Riboswitches are gene regulatory elements that are frequently found in the 5′-untranslated regions of bacterial mRNAs (1–6). Only very recently, the nadA RNA motif has been assigned to function as a riboswitch which regulates the expression of genes involved in biosynthesis of the enzyme cofactor nicotinamide adenine dinucleotide (NAD+). Although the cofactor is ubiquitous, this riboswitch appears to be rather rare and has the special feature of a tandem aptamer architecture. Here, we report crystal structures of the first, as well as the second domain of the NAD+ riboswitch, both individually bound to NAD+.

For the structural studies on domain 2 of the NAD+ riboswitch, we used the sequence information from Acidobateriaceae bacterium KBS83. Though attempts to crystallize the full-length NAD+ riboswitch in the presence of NAD+ were unsuccessful, we did succeed in generating crystals of domain 2 alone in complex with NAD+ (832GAAA-D2/NAD+), diffracting at a resolution of 2.1 Å. The structure was named as 832GAAA-D2/NAD+, the space group of 832GAAA-D2/NAD+ was P3221, in which each asymmetric unit contain one molecule. Also, the ligand NAD+ is bound similarly to domain 1, positioned at the intersection of the north terminus of stem P1 and the junction J1. All stacking and hydrogen bonding interactions are retained and the three octahedrally coordinated Mg2+ ions are also present with a similar coordination pattern to NAD+ and the nucleotides in the binding pocket of 832GAAA-D2. The long double helical arrangement of stem P1a and P1b, however, shows clear distinctions originating from the altered nucleoside composition of J2 in 832GAAA-D2 that comprises only four instead of the original 6 nt. G23 forms a Watson–Crick base pair with C37 in J2 of 18GAAA-D1, however, the corresponding nucleotides G23 and U35 in 832GAAA-D2 do not pair, but form a non-planar base triple interaction with G34. It is notable that G34 from 832GAAA-D2, whose corresponding nucleotide is G36 in 18GAAA-D1, does not exhibit the long-distance interaction with C14 in J1, but points inwards and interacts with G23-G34-U35 instead. Furthermore, G36 in 832GAAA-D2, whose corresponding nucleotide is G38 in 18GAAA-D1, also lacks the long-distance pairing to J1 but forms a Watson–Crick base pair with C12′ from a symmetric molecule in the crystal, resulting in symmetry-related dimers of 832GAAA-D2.

> GGUUUCAACAUCCCCGUUCGGCGCUCGAAAGAGGUGGCCGGACUGAAGCC>[2x]MMVGDGIAKFIPEGFDAQKIPSFAIEKEPREQGALPADWVLVPEFSLTDGKANASLTVPEGTSIYGGGEVTGSLLRNGKTIKLWNTDSGAYGVDKGTRLYQSHPWMMGVRKDGTAFGILFDTTWKAELSSTDEKIELKSEGIPFRVFIIDRESPQAVIRGLSELT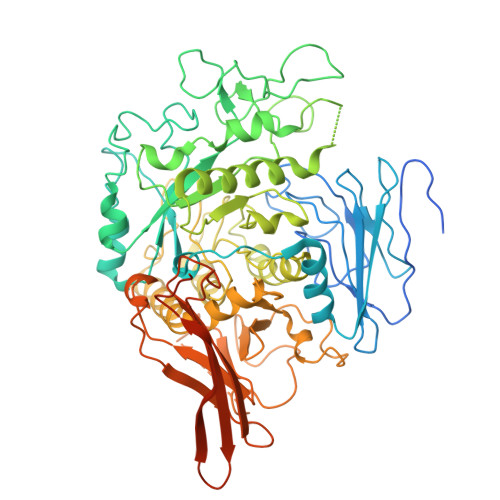GTMPMIPRWALGYQQCRFSYSPDSRVIEIADTFRLKRIPCDVIWMDIDYMDGYRIFTFNPKSFPNPKAVNRDLHIRGFHSAWMIDPGAKVDPNYFVYKSGTENDVWVKTADGKNFHGDAWPGAAAFPDFTSPKVNKWWRNLYKDFLAQGVDGVWNDVNEPQINDTPNKTMPEDNLHRGGGKLPAGTHLQYHNVYGFLMVKASREGILDARPEKRPFILTRSNFLGGQRYAATWTGDNGSCWDHLKMSVPMSLTLGLSGQPFSGADIGGFLFNADADLFGNWIGFGAFYPFARGHACAGTNNKEPWVFGQKVEDASRIALERRYILLPYFYTLLHEASTNGMPIMRPVFFSDPKDLSLRAEEEAFLVGDNLLIIPAFANQPALPKGIWKELSLVEGDQNDKYQAKMKIRGGAIIPTGKIIQNTTENSLDPLTLLVCLDEQGKASGNMYWDAGDGWSYKKGDYSLLQFVAERNGDKVTVKLTKKTGKYNTENKDMAVIKIITDQGIRQASGNLVEGIEIRLHHHHHHLRVPRGS> MDILENYVSFDEQARDINIAFDKLFGRDDISHMNN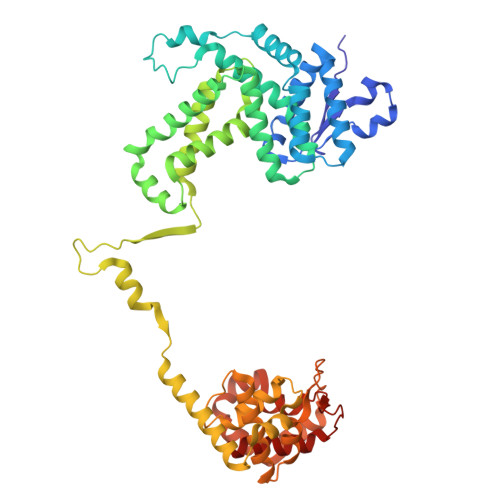FSINKRSYYNCLDQISDDLNLVLNKYNDLAYSLLEIRYNMATKENYTHMEFYSDIERLFIKNEKLLNVISDIVEEEYDLDLNQASKGKKINIELQVTDNLNKIYLKSSVLMRILIPILCDFNCDDDINEVLVYDIFKEVIKSFDDGKKNALNKLYKIIYSRVFETKYSDVVIWTYLKNMSTDLMIIVKDYFKVIIKKIFPKLKHNSSVISYLDVVIKQKLKYLFTFKYPISYKPLKAETTDDEELSEQERMEINLLRNDQGNSIINECSIKQEIAKIKKKYNVTDEVMKEFINGRELNSIQIYLVKIYYSNKFKVNSNKNDIFYLLYGMTRELGEMNFSIIPEILSCAIAPNVRKMNNRKKLVDKIIHSDKYSYLLKSYLPIKNILDKNNVILQLMTIKNAKFMNKENKEVDFSTDHLAEEVLDMLLCI>[2x]GHMNAAPNRNLFDRVLHGQAPCFALIARSTGSAGERAMIDVFAGAVSYPSSLAELPLAAPTATGADRQELLVMVPYRQLHERGFKTHDDGAPLVAITCDEHETVSAQLALAAIPDADTALGERHFDIDDEAYAEIVERVITDEIGTGAGSNFVIKRTLEGDLDDYSPAKALAVFKRLMRREVGAYWIFVIHTGER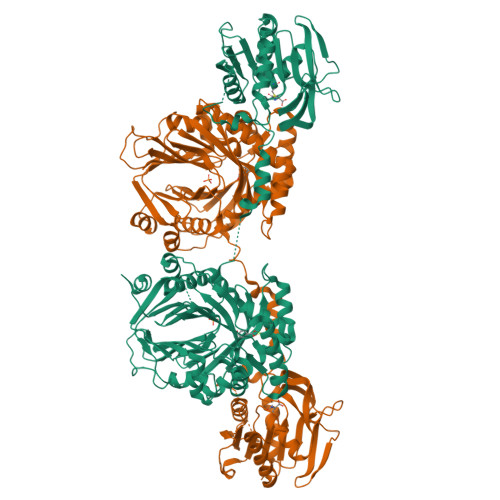TFVGATPERHLTLHEGCATMNPISGTYRYPQSGPTIDGINAFLGDRKESDELYMVLDEELKMMARICPAGGQVTGPHLREMARLAHTEYFIVGHTEADVRDLLRETMFAPTVTGSPIESATRVIARHERAGRGYYSGIAALIGRDARGGRTLDSAILIRTAEIDRAGHVRIGVGSTLVRHSDAVSEVMETHAKVAALSNAFDPPEAGPALGQHPSVQAALRERNEGIADFWFRPYGGRQGEMADELAELSGCRALIVDAEDHFTAMIAQQLSSLGLATEVCGVHDAVDLARYDVVVMGPGPGDPSDAGDPRIARLYAWLRHLIDEGKPFMAVCLSHQILNAILGIPLVRREVPNQGIQVEIDLFGQRERVGFYNTYVAQTVRDEMDVDGVGTVAISRDPRTGEVHALRGPTFSSMQFHAESVLTVDGPRILGEAITHAIRREKRMTALTA>GMKMLEQLEKKL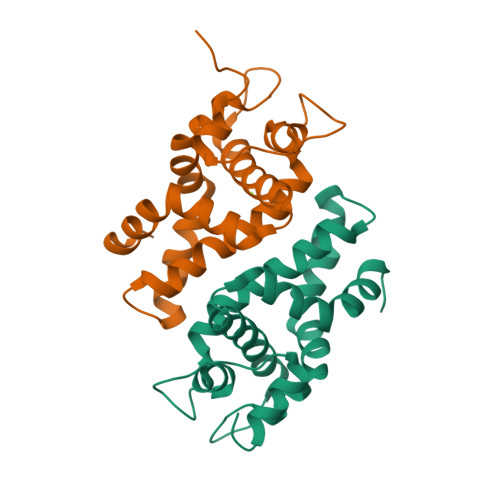GYTFKDKSLLEKALTHVSYSKKEHYETLEFLGDALVNFFIVDLLVQYSPNKREGFLSPLKAYLISEEFFNLLAQKLELHKFIRIKRGKINETIIGDVFEALWAAVYIDSGRDANFTRELFYKLFKEDILSAIKEGRHHHHHH[4x]>MGSSHHHHHHSSGRENLYFQSMSRVSHEQFRAALQLVVSPGDPREYLANFIKIGEGSTGIVCIATEKHTGKQVAVKKMDLRKQQRRELLFNEVVIMRDYHHDNVVDMYSSYLVGDELWVVMEFLEGGALTDIVTHTRMNEEQIATVCLSVLRALSYLHNQGVIHRDIKSDSILLTSDGRIKLSDFGFCAQVSKEVPKRKSLVGTPYWMAPEVISRLPYGTEVDIWSLGIMVIEMIDGEPPYFNEPPLQAMRRIRDSLPPRVKDLHKVSSVLRGFLDLMLVREPSQRATAQELLGHPFLKLAGPPSCIVPLMRQYRHH[2x]

PAKs are serine/threonine protein kinases that are regulated by Rho GTPases of the Cdc42 and Rac families (Knaus et al., 1995; Manser et al., 1994; Martin et al., 1995). In humans, the PAK family comprises six members, which are classified into groups I (PAK1, -2, and -3) and II (PAK4, -5, and -6) based on their domain architecture and regulatory properties (Bokoch, 2003; Jaffer and Chernoff, 2002; Kumar et al., 2006; Zhao and Manser, 2005). Group II PAKs (PAK4–6) regulate a wide variety of cellular functions, and PAK deregulation has been linked to tumor development. Comparison of five high-resolution crystal structures comprising the kinase domains of all three monophosphorylated, enzymatically active group II PAK family members revealed a number of catalytically productive and nonproductive conformers presumably representing snapshots of catalytic domain movements during catalysis.

In order to elucidate the molecular mechanisms of inhibition, we determined the structures of a 2, 6, 9-trisubstituted purine inhibitor (N-(cis-2-Aminocyclohexyl)-N-(3-chlorophenyl)-9-ethyl-9H-purine-2, 6-diamine) with PAK4 and PAK5. Interestingly, PAK5 crystallized with two molecules in the asymmetric unit; one molecule was found in a noncatalytically productive conformation with an unoccupied active site (apo-PAK5), and the other bound the purine inhibitor and was in a closed, catalytically productive conformation. The detailed mechanism for the group II PAKs was best highlighted by the structure of PAK5 complexed with the purine inhibitor. In this crystal, the asymmetric unit accommodated two molecules, only one of which had the purine bound, allowing the comparison of a catalytically productive, inhibitor-bound conformation with an open, catalytically nonproductive apo structure under identical crystallization conditions. In PAK5, the phosphorylated Ser602 forms a hydrogen bond network with Arg600, Arg567, Tyr620, and Phe589. This hydrogen bond network links both ends of the activation segment via the catalytic loop residue Arg567. In the PAK5 inhibitor complex, the last turn of the αC helix is distorted and becomes a loop region, thus adding length to the αC–β4 loop. In contrast, the N terminus of αC gains an additional turn with the rearrangement of the βC–αC loop. In the PAK5 purine complex, the αC N-terminal extension leads to the formation of two hydrogen bonds, between the conserved αC Arg487 and main chain residues of the glycine-rich loop residues Ser459 and Gly458, respectively, as well as the formation of a salt bridge by the carboxyl group of Glu457. In the catalytically nonproductive PAK5 apo structure, Arg487 is disordered after the γ carbon.> MNLRAAGPGWLFCPADAPEAFAAAAAAADVVILDLEDGVAAAQKPAARNALRDTPLDPERTVVRINAGGTADQARDLEALAGTAYTTVMLPKAESAAQVIELAPRDVIALVETARGAVCAAEIAAADP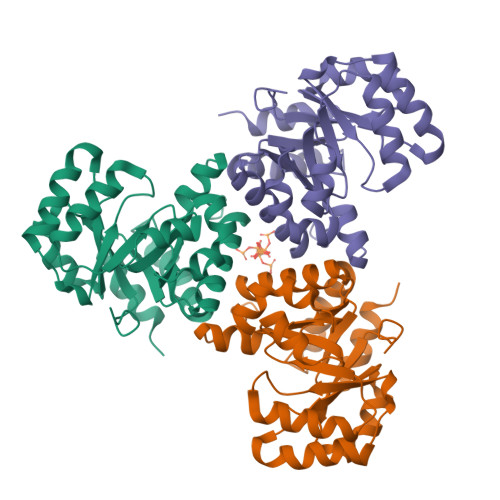TVGMMWGAEDLIATLGGSSSRRADGAYRDVARHVRSTILLAASAFGRLALDAVHLDILDVEGLQEEARDAAAVGFDVTVCIHPSQIPVVRKAYAASHEKLAWARRVLAASRSERGAFAFEGQMVDSPVLTHAETMLRRAGEATSE> DKRAHHNALERKRR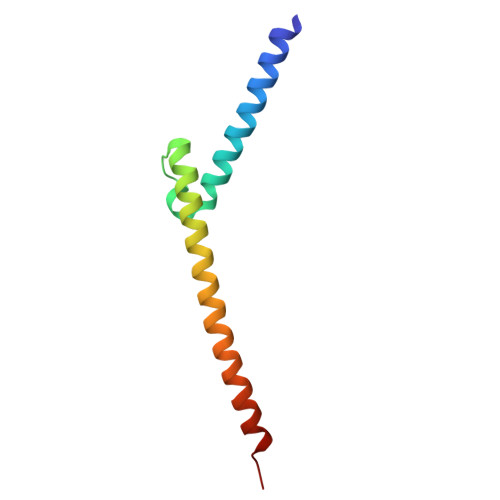DHIKDSFHSLRDSVPSLQGEKASRAQILDKATEYIQYMRRKNHTHQQDIDDLKRQNALLEQQVRALGGC>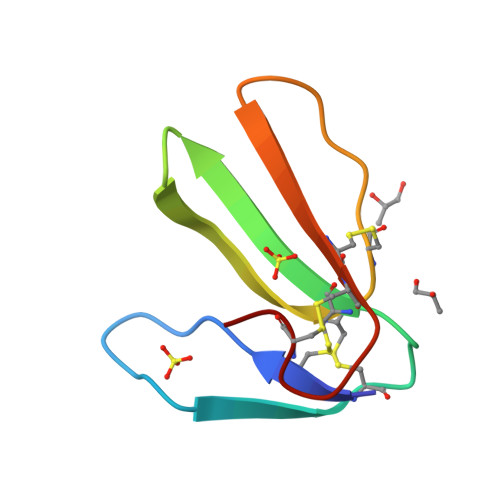[3x]TICHIQISKTHGILKTCEENSCYKMSVRGWIIGRGCGCPSAVRPRQVQCCTSDKCNY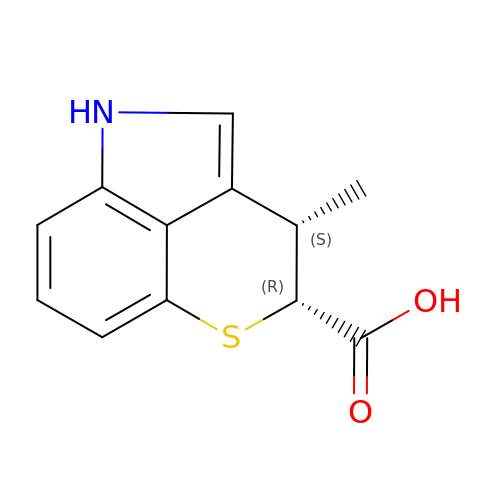(5~{S},6~{R})-5-methyl-7-thia-2-azatricyclo[6.3.1.0^{4,12}]dodeca-1(12),3,8,10-tetraene-6-carboxylic acid | C12 H11 N O2 S | DKHFLDXCKWDVMF-UPONEAKYSA-N Src homology 2 domain-containing inositol phosphate phosphatase 2 (SHIP2) is one of the 10 human inositol phosphate 5-phosphatases. One of its physiological functions is dephosphorylation of phosphatidylinositol 3,4,5-trisphosphate, PtdIns(3,4,5)P3. It is therefore a therapeutic target for pathophysiologies dependent on PtdIns(3,4,5)P3 and PtdIns(3,4)P2. Therapeutic interventions are limited by the dearth of crystallographic data describing ligand/inhibitor binding.

Finally, using a structural biology approach, we solve the structure of a SHIP2 catalytic domain in complex with a bound dimeric ligand and potent inhibitor. The related compound, 5,5′-ethane-1,2-diylbis(oxy)bis(benzene-1,2,4-trisphosphate)20 (5) (hereafter named 1,2,4-dimer), is a bridged dimer of the surrogate ligand of IP3Rs, benzene 1,2,4-trisphosphate. The crystal structure of the 1,2,4-dimer-SHIP2cd complex comprises two monomers of SHIP2 and a single copy of the inhibitor in the asymmetric unit. The 1,2,4-dimer does not occupy the positions of the crystallographically resolved ligands or of the predicted bound states of docked ligands in catalytic domain or multidomain structures. Indeed, the 1,2,4-dimer ligand fails to directly contact the L4 loop. Remarkably, we observe that phosphate P4 of 1,2,4-dimer interacts with D613. This, we suggest, precludes interaction of this residue with R682 and adoption of the L4-out conformation that, in its transient motions, accompanies optimal catalysis. While the distal binding of 1,2,4-dimer does not significantly modify the L4 closed (L4-in) conformation from that seen in the complex with BiPh(2,3′,4,5′,6)P5 (1), the compound is a potent displacer of 2-FAM-InsP5 and a potent inhibitor of 5-phosphatase activity against Ins(1,3,4,5)P4. Thus, 1,2,4-dimer meets both the kinetic and structural criteria of an uncompetitive allosteric inhibitor of SHIP2. One intriguing possibility is that a previously unrecognized substrate or product is evident in the 1,2,4-dimer (5)-liganded structure.

>[2x]SMDEPDMISVFIGTWNMGSVPPPKNVTSWFTSKGLGKTLDEVTVTIPHDIYVFGTQENSVGDREWLDLLRGGLKELTDLDYRPIAMQSLWNIKVAVLVKPEHENRISHVSTSSVKTGIANTLGNKGAVGVSFMFNGTSFGFVNCHLTSGNEKTARRNQNYLDILRLLSLGDRQLNAFDISLRFTHLFWFGDLNYRLDMDIQEILNYISRKEFEPLLRVDQLNLEREKHKVFLRFSEEEISFPPTYRYERGSRDTYAWHKQKPTGVRTNVPSWCDRILWKSYPETHIICNSYGCTDDIVTSDHSPVFGTFEVGVTSQ>SNAMDKKIIGIDLGGTTIKFAILTTDGVVQQKWSIETNILEDGKHIVPSIIESIRHRIDLYNMKKEDFVGIGMGTPGSVDIEKGTVVGAYNLNWTTVQPVKEQIESALGIPFALDNDANVAALGERWKGAGENNPDVIFITLGTGVGGGIVAAGKLLHGVAGCAGEVGHVTVDPNGFDCTCGKRGCLETVSSATGVVRVARHLS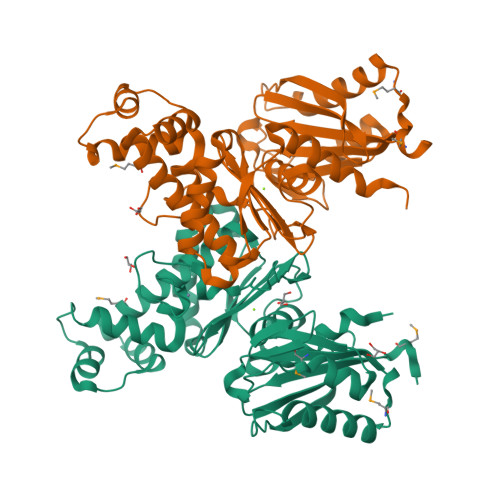EEFAGDSELKQAIDDGQDVSSKDVFEFAEKGDHFALMVVDRVCFYLGLATGNLGNTLNPDSVVIGGGVSAAGEFLRSRVEKYFQEFTFPQVRNSTKIKLAELGNEAGVIGAASLALQFSKEK[4x]In this study, we determined the crystal structures of E. coli (S)-ureidoglycolate dehydrogenase AllD, which forms oxalurate in the presence of NAD+. This structure represents a metabolic branch point enzyme during (S)-ureidoglycolate utilization, which is the end product of purine catabolism common to plants, as well as some bacteria and fungi. (S)-Ureidoglycolate dehydrogenase AllD belongs to one of eight clades of l-sulfolactate dehydrogenase-like superfamily. The dimeric structure observed in the asymmetric unit represents the functional unit of AllD, consistent with size-exclusion chromatography, in which AllD eluted as a dimer.

The structure for the binary complex of AllD with NADH (the AllD–NADH complex) revealed a binding pocket for a cofactor NADH which is localized mainly at the inter-domain interface of each subunit, and further stabilized by dimerization. Specifically, NADH adopts an extended conformation and is located on top of the central β-sheet of Domain II, with its orientation perpendicular to that of the β-strands. The nicotinamide ring faces toward the inner side of monomer, while the adenine moiety is located at the intersubunit interface. NADH is buried in the pocket such that only 10% of the possible surface area is exposed. In particular, the nicotinamide ring, which acts as a hydride acceptor or donor during catalysis, is located on top of the N-terminus of β8, and its position appears to be stabilized by stacking interactions between Pro158 and His44, with further adjustments by hydrogen bonding between its carbonyl and amino group to His116 and Ser140, respectively. Notably, the pro-S face at C4 (i.e. B-face) of the nicotinamide ring is exposed to and accessible from the solvent, suggesting that this face functions as the putative substrate-binding site. Specifically, in the binary complex, binding of NADH into the active site caused a rigid-body movement of Domain III toward Domain II at the inter-domain interface; residues Val179 to Ser194 containing a helix α6 in Domain III showed large displacements of Cα atoms in the range of 0.9–3.0 Å. Compared to the apo structure, the side chain of His44 moved out by 1.2 Å, accommodating NADH and forming a possible stacking interaction with the nicotinamide ring, while Asp174 rotated its side chain as much as 4.0 Å toward NADH and hydrogen bonded with the hydroxyl group of ribose, adjacent to the nicotinamide ring. Additionally, the carboxylate group of Asp308 moved approximately 1.0 Å, forming a hydrogen bond with the hydroxyl group of ribose adjacent to the adenine base. In addition, the NADH cofactor adopts an extended conformation, which is clearly distinguishable from a bent conformation usually associated with other NAD(P)H-dependent oxidoreductases.

>GHMKISRETLHQLIENKLCQAGLKREHAATVAEVLVYADARGIHSHGAVRVEYYAERISKGGTNREPEFRLEETGPCSAILHADNAAGQVAAKMGMEHAIKTAQQNGVAVVGISRMGHSGAISYFVQQAARAGFIGISMCQSDPMVVPFGGAEIYYGTNPLAFAAPGEGDEILTFDMATTVQAWGKVLDARSRNMSIPDTWAVDKNGVPTTDPFAVHALLPAAGPKGYGLMMMIDVLSGVLLGLPFGRQVSSMYDDLHAGRNLGQLHIVINPNFFSSSELFRQHLSQTMRELNAITPAPGFNQVYYPGQDQDIKQRKAAVEGIEIVDDIYQYLISDALY[2x]pmcHuman ornithine aminotransferase (hOAT) is an enzyme that catalyzes the transfer of the δ-amino group from l-ornithine (l-Orn) to α-ketoglutarate (α-KG). As a pyridoxal-5′-phosphate (PLP)–dependent transaminase, hOAT has a “Bi−Bi, Ping–Pong” kinetic mechanism. In the first half-reaction, PLP and l-Orn are converted to pyridoxamine phosphate (PMP) and l-glutamate-γ-semialdehyde (l-GSA). l-GSA is then prone to cyclize to Δ1-pyrroline-5-carboxylate (P5C). In the second half-reaction, hOAT catalyzes the transfer of the amino group of PMP to an α-keto acid, preferentially α-KG, forming glutamate and regenerating the PLP form of the cofactor.

The structure of hOAT crystal soaked with AVA revealed an intermediate that closely resembles the gem–diamine intermediate. Unlike other intermediates in a typical transamination reaction, the gem–diamine is an early intermediate in which the catalytic lysine, the PLP, and the substrate are covalently joined together, and the observed electron density can be fit convincingly to such an intermediate state. The carboxylate group of AVA formed a strong hydrogen bond (measured as 2.2 Å) with Tyr55 and indirectly interacted with Arg180 through hydrogen bonds via a water molecule, and the Glu235–Arg413 salt bridge remained intact. That this intermediate is observed in the crystal indicates that the lattice greatly modifies the magnitude and relative rates of the chemistry, in that no evidence for a gem–diamine species was observed for the same reaction in solution. Internal aldimine and gem–diamine were found anchored by the side chain of catalytic Lys292 tilting the pyridine ring of PLP. Thus, the observed AVA gem–diamine intermediate is likely resulted from a trapping effect during crystal soaking. To the best of our knowledge, this is the first experimentally observed gem–diamine structure among all hOAT substrates. Of all chemical species present in crystallization condition, only the phosphate group of PLP possesses the right geometry to fit into the observed electron density. The electron density observed in the Ser186–Met201–Phe204 site likely represents a PLP bound only as a crystallographic artifact.

>MFSKLAHLQRFAVLSRGVHSSVASATSVATKKTVQGPPTSDDIFEREYKYGAHNYHPLPVALERGKGIYLWDVEGRKYFDFLSSYSAVNQGHCHPKIVNALKSQVDKLTLTSRAFYNNVLGEYEEYITKLFNYHKVLPMNTGVEAGETACKLARKWGYTVKGIQKYKAKIVFAAGNFWGRTLSAISSSTDPTSYDGFGPFMPGFDIIPYNDLPALERALQDPNVAAFMVEPIQGEAGVVVPDPGYLMGVRELCTRHQVLFIADEIQTGLARTGRWLAVDYENVRPDIVLLGKALSGGLYPVSAVLCDDDIMLTIKPGEHGSTYGGNPLGCRVAIAALEVLEEENLAENADKLGIILRNELMKLPSDVVTAVRGKGLLNAIVIKETKDWDAWKVCLRLRDNGLLAKPTHGDIIRFAPPLVIKEDELRESIEIINKTILSF[3x]>[2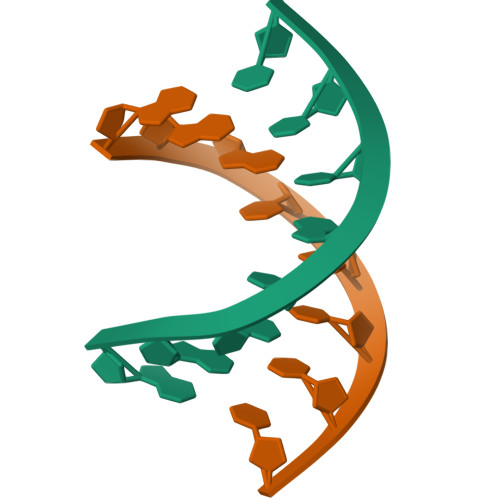x]GGGTGCCC>MISLQSDQLLEATVGQFMIEADKVAHVQVGNNLEHALLVLTKTGYTAIPVLDPSYRLHGLIGTNMIMNSIFGLERIEFEKLDQITVEEVMLTDIPRLHINDPIMKGFG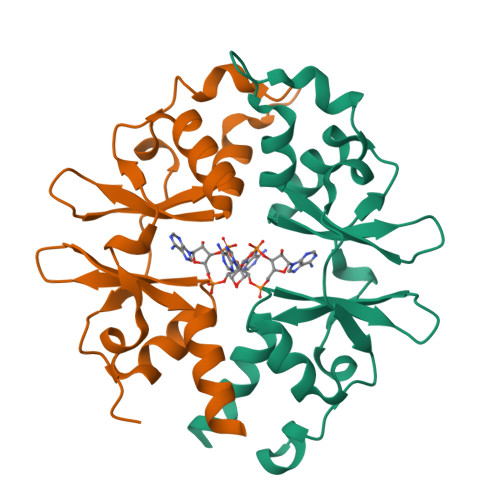MVINNGFVCVENDEQVFEGIFTRRVVLKELNKHIRSLNK[2x]>MAAPARDPPGYRYAAAILPTGSILSTIEVASHRRLFDFFAAVRSDENSLYDVEFDALLGSYCNTLSLVRFLELGLSVACVCTKFPELAYMNEGRVQFEVHQPLIARDGPHPVEQPVHNYMTKVIDRRALNAAFSLATEAIALLTGEALDGTGISLHRQLRAIQQLARNVQAVLGAFERGTADQMLHVLLEKAPPLALLLPMQRYLDNGRLATRVARATLVAELKRSFCDTSFFLGKAGHRREAIEAWLVDLTTATQPSVAVPRLTHADTRGRPVDGVLVTTAAIKQRLLQSFLKVEDTEADVPVTYGEMVLNGANLVTALVMGKAVRSLDDVGRHLLDMQEEQLEANRETLDELESAPQTTRVRADLVAIGDRLVFLEALERRIYAATNVPYPLVGAMDLTFVLPLGLFNPAMERFAAHAGDLVPAPGHPEPRAFPPRQLFFWGKDHQVLRLSMENAVGTVCHPSLMNIDAAVGGVNHDPVEAANPYGAYVAAPAGPGADMQQRFLNAWRQRLAHGRVRWVAECQMTAEQFMQPDNANLALELHPAFDFFAGVADVELPGGEVPPAGPGAIQATWRVVNGNLPLALCPVAFRDARGLELGVGRHAMAPATIAAVRGAFEDRSYPAVFYLLQAAIHGNEHVFCALARLVTQCITSYWNNTRCAAFVNDYSLVSYIVTYLGGDLPEECMAVYRDLVAHVEALAQLVDDFTLPGPELGGQAQAELNHLMRDPALLPPLVWDCDGLMRHAALDRHRDCRIDAGGHEPVYAAACNVATADFNRNDGRLLHNTQARAADAADDRPHRPADWTVHHKIYYYVLVPAFSRGRCCTAGVRFDRVYATLQNMVVPEIAPGEECPSDPVTDPAHPLHPANLVANTVKRMFHNGRVVVDGPAMLTLQVLAHNMAERTTALLCSAAPDAGANTASTANMRIFDGALHAGVLLMAPQHLDHTIQNGEYFYVLPVHALFAGADHVANAPNFPPALRDLARDVPLVPPALGANYFSSIRQPVVQHARESAAGENALTYALMAGYFKMSPVALYHQLKTGLHPGFGFTVVRQDRFVTENVLFSERASEAYFLGQLQVARHETGGGVNFTLTQPRGNVDLGVGYTAVAATGTVRNPVTDMGNLPQNFYLGRGAPPLLDNAAAVYLRNAVVAGNRLGPAQPLPVFGCAQVPRRAGMDHGQDAVCEFIATPVATDINYFRRPCNPRGRAAGGVYAGDKEGDVIALMYDHGQSDPARPFAATANPWASQRFSYGDLLYNGAYHLNGASPVLSPCFKFFTAADITAKHRCLERLIVETGSAVSTATAASDVQFKRPPGCRELVEDPCGLFQEAYPITCASDPALLRSARDGEAHARETHFTQYLIYDASPLKGLSL[6x];>MITDCFEADIAIPSGISRPDAAALQRCEGRVVFLPTIRRQLALADVAHESFVSGGVSPDTLGLLLAYRRRFPAVITRVLPTRIVACPVDLGLTHAGTVNLRNTSPVDLCNGDPVSLVPPVFEGQATDVRLESLDLTLRFPVPLPTPLAREIVARLVARGIRDLNPDPRTPGELPDLNVLYYNGARLSLVADVQQLASVNTELRSLVLNMVYSITEGTTLILTLIPRLLALSAQDGYVNALLQMQSVTREAAQLIHPEAPMLMQDGERRLPLYEALVAWLAHAGQLGDILALAPAVRVCTFDGAAVVQSGDMAPVIRYP[2x];> MKTKPLPTAPMAWAESAVETTTSPRELAGHAPLRRVLRPPIARRDGPVLLGDRAPRRTASTMWLLGIDPAESSPGTRATRDDTEQAVDKILRGARRAGGLTVPGAPRYHLTRQVTLTDLCQPNAERAGALLLALRHPTDLPHLARHRAPPGRQTERLAEAWGQLLEASALGSGRAESGCARAGLVSFNFLVAACAAAYDARDAAEAVRAHITTNYGGTRAGARLDRFSECLRAMVHTHVFPHEVMRFFGGLVSWVTQDELASVTAVCSGPQEATHTGHPGRPRSAVTIPACAFVDLDAELCLGGPGAAFLYLVFTYRQCRDQELCCVYVVKSQLPPRGLEAALERLFGRLRITNTIHGAEDMTPPPPNRNVDFPLAVLAASSQSPRCSASQVTNPQFVDRLYRWQPDLRGRPTARTCTYAAFAELGVMPDDSPRCLHRTERFGAVGVPVVILEGVVWRPGGWRACA;>[6x]MAAPQFHRPSTITADNVRALGMRGLVLATNNAQFIMDNSYPHPHGTQGAVREFLRGQAAALTDLGVTHANNTFAPQPMFAGDAAAEWLRPSFGLKRTYSPFVVRDPKTPSTP

Here we show asymmetric reconstructions of herpes simplex virus 2 (HSV-2) B- (containing scaffold proteins inside, putative capsid assembly intermediate), C- (DNA-filled capsid, derived from the enveloped virion by using detergent treatment to remove viral membrane proteins and outer tegument proteins) and virion-capsids (enveloped intact virion) at 8.1, 9.0 and 10.2 Å respectively. The asymmetric reconstructions reveal a unique portal vertex in the context of the icosahedral capsid, including 1 portal, 11 pentons, 3 types of hexons (P, peripentonal; E, edge; C, center) with the hexameric rings formed by VP26s, 320 triplexes (Ta-Tf) and 12 pentagram-shaped capsid vertex specific component (CVSC) densities (composed of a UL17 monomer, a UL25 dimer and a UL36 dimer, presence in C- and virion-capsids). Radially colored representations of the three reconstructions reveal the dodecameric portal situated beneath one of the pentameric vertices; but, the density surrounding the portal displays a five-fold symmetrical assembly, highlighting the symmetry-mismatch structural features. The portal vertex of the capsid is a hub for protein-protein interactions that are important for capsid assembly and genome packaging.

When five-fold symmetry was imposed, the resolution of local reconstructions for the portal vertex in B-, C- and virion-capsids was improved to 4.05, 4.50 and 5.36 Å, respectively, albeit that the portal was five-fold averaged. The presence of scaffold proteins, some of which possibly associate with the portal, is observed in the B-capsid. Apart from the lack of the CVSC, PVAT and genome in the B-capsid and conformational differences on the portal as well as PVAT, the structures of the three capsids are indistinguishable. A comparison of asymmetric reconstructions of the portal vertex of the three capsids reveals notable differences in the position and morphology of the portal and PVAT. Strikingly, the portal in the B-capsid situates inwards by ~30 Å. It exposes itself by lacking the PVAT and forms a basin at the portal vertex, suggesting a ready-state for docking of terminase complexes and genome packaging, when compared to those in the C- or virion-capsids. Interestingly a novel network of subunit contacts is observed between the portal and PV-Ta and varies each other in three capsids. Lying on the portal head, a novel five-fold symmetrical assembly comprising five copies of a well-resolved two-helix coiled coil (presumably being the fragment from the portal or pUL36) shows close contacts with PV-Ta. The N-lasso in PVP1 refolds from a β-strand-rich structure into two helices, resulting in a loss of its lassoing ability, whilst PVP6 dimerization domain moves from nearby the E-loop to the central helix abrogating the two-fold interactions.(1S)-1-AMINO-2-(1H-INDOL-3-YL)ETHANOL 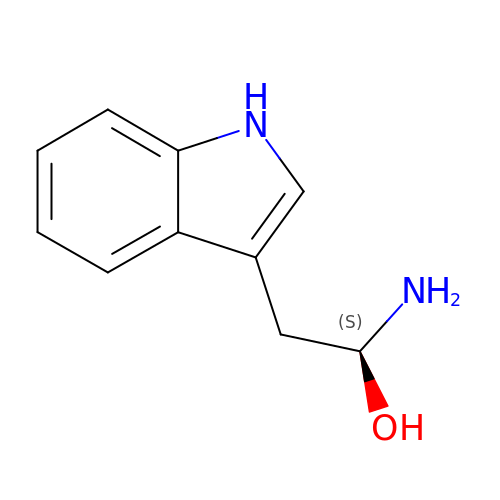| C10 H12 N2 O | WNWJSYYPDDQIQV-JTQLQIEISA-N>GTKRPFRQNLNPLVLLLDAALTGELEVVQQAVKEMNDPSQPNEEGITALHNAICGANYSIVDFLITAGANVNSPDSHGWTPLHCAASCNDTVICMALVQHGAAIFATTLSDGATAFEKCDPYREGYADCATYLAD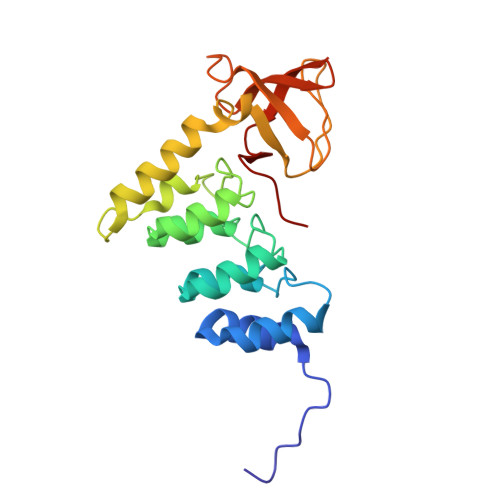VEQSMGLMNSGAVYALWDYSAEFGDELSFREGESVTVLRRDGPEETDWWWAALHGQEGYVPRNYFGLFPRVKPQR[4x]> ALPQTVRIGTDTTYAPFSSKDAKGEFIGFDIDLGNEMCKRMQVKCTWVASDFDALIPSLKAKKIDAIISSLSITDKAQQEIAFSDKLYAADSRLIAAKGSPIQPTLESLKGKHVGVLQGSTQEAYANDNWRTKGVDVVAYANQDLIYSDLTAGRLDAALQDEVAASEGFLKQPAGKEYAFAGPSVKDKKYFG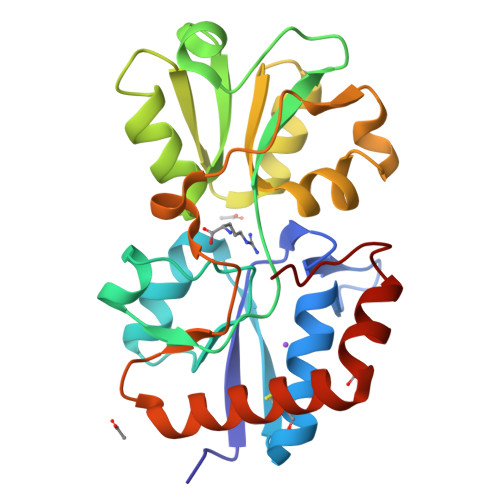DGTGVGLRKDDTELKAAFDKALTELRQDGTYDKMAKKYFDFNVYGD>[3x]MDSKQQRIGVIGTGAIGG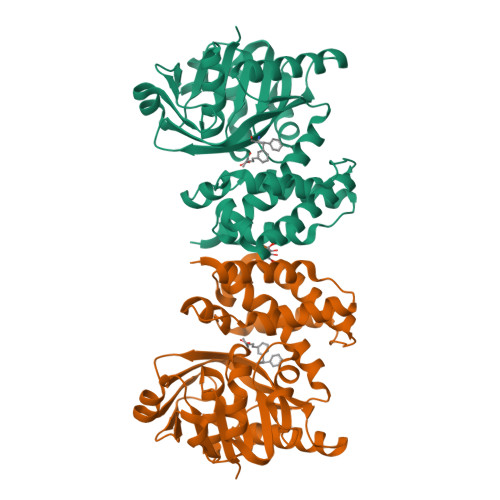FYGLMLAHAGHDVHFLLRSEFEAVNRAGLSLNSAVHGFRRLAPVQAYHSAQDMPPCDWLLVGAKTTGNHELAPLIRAAAAPGAKVLLLQNGLGVEERLRPLLPESLHLLGGLCFICVHRGEPGVIEHQAYGGVNLGYHSGPADERRRREIVEEGAALFRESGLESTAMPDLEQARWQKLVWNIPYNGLSVLLKSSTAPLMANADSRSLIEAIMEEVIGAAGACGFILPEGYADQLLAATERMPDYRPSMYHDFAHGRPLELAAIYAAPLARAAAAGYRMPRVEALHQALRFLEAQPR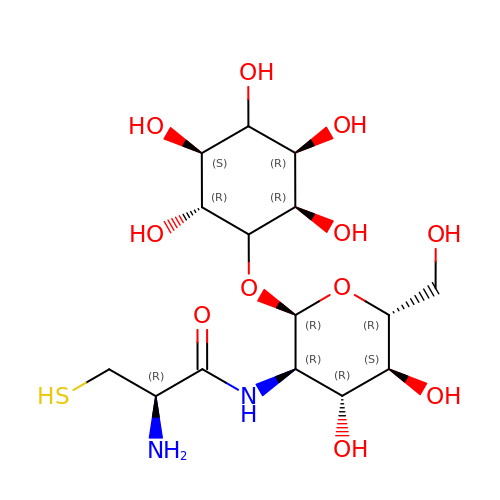(1S,2R,3R,4S,5S,6R)-2,3,4,5,6-pentahydroxycyclohexyl 2-(L-cysteinylamino)-2-deoxy-alpha-D-glucopyranoside | C15 H28 N2 O11 S | ZGXSCMBZZVXWGF-BSEFFJTHSA-N> GSSRAMGNEVAGVEDISVEITPSSKRNSDARRTSRNCSSNEERKRRKYFHMLYLVCLMVHGFIRNEWINSKRLSRKLSNLVPEKVFELLHPQKDEELPLRSTRKLLDGLKKCMELWQKHWKITKKYDNEGLYMRTWKEIEMSANNKRKFKTLKRSDFLRAVSKGHGDPDISVQGFVAMLRACNVNARLIMSCQPPDFTNMKIDTSLNGNNAYKDMVKYPIFWCEVWDKFSKKWITVDPVNLKTIEQVRLHSKLAPKGVACCERNMLRYVIAYDRKYGCRDVTRRYAQWMNSKVRKRRITKDDFGEKWFRKVITALHHRKRTKIDDYEDQYFFRRDESEGIPDSVQDLKNHPYYVLEQDIKQTQIVKPGCKECGYLKVHGK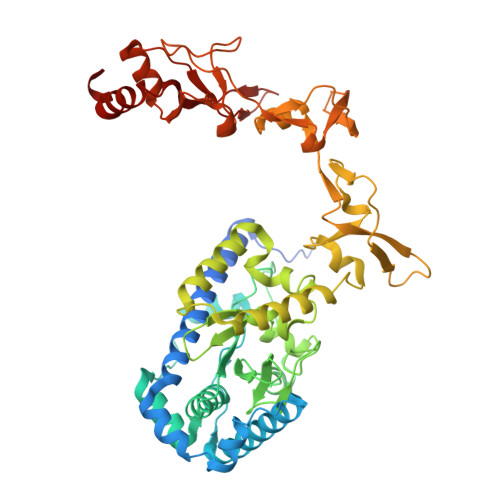VGKVLKVYAKRDIADLKSARQWYMNGRILKTGSRCKKVIKRTVGRPKGEAEEEDERLYSFEDTELYIPPLASASGEITKNTFGNIEVFAPTMIPGNCCLVENPVAIKAARFLGVEFAPAVTSFKFERGSTVKPVLSGIVVAKWLREAIETAIDGIEFI> MVNNINWVKLPVILDRLLRHPLLTDLNLETAIQYTLDFISAMGLPNVY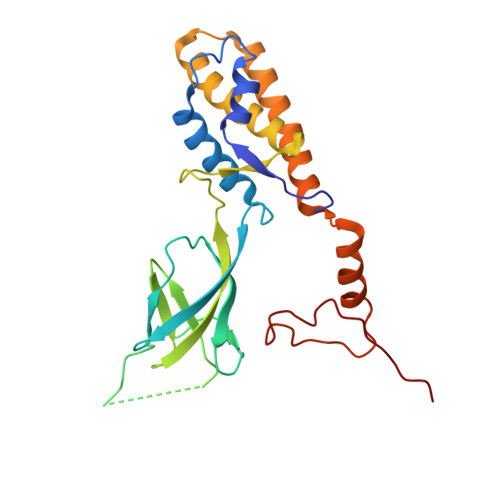VDKIETIDIKEYRGELPCDLISINQVRLHKNGIALRAMTDNFNAYPTHDHKEGDWYERGEPSFKTQGRVIFTSIKHEKVDISYKAIMLDDEGLPLIPDNPIFLKTLELYIKKEWFTILFDMGKISPAVLNNTQQEYAFKAGQCNNEFVIPSVSEMEAITNMWNQLIPRVTEFRRGFKNLGDKEYIRVH> KTNENVISFFDSTDAETQNHDVLMKGCGEFIVNLRTLLRTFRTITDNWILQANTKTPITDLTNTTDAQGRDYMSYLSYLYRFYRGGRRYKFFNTTPLKQSQTCYIRSFLMPRNYSADEINVDGPSHITYPVINPVHEVEVPFYSQYRKIPIASTSDKGYDSSLMYFSNTSTTQIVARAGNDDFTFGWMIGPPQLQGETRSVVP;> KPRNQQQVCPLQNVPAWGYSLYKGIDMSVPLAYDPNNELGDLKDVFPSAVDEMAIGYVCGNPAVKHV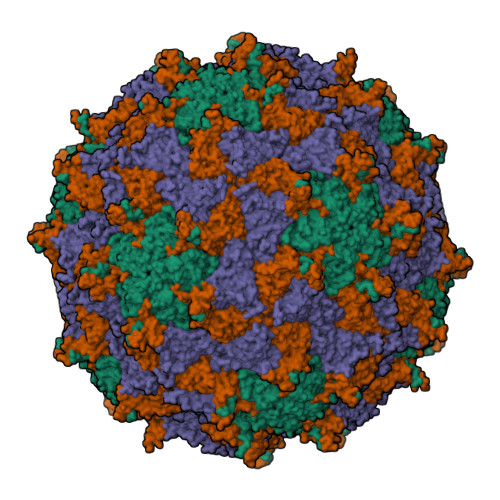LTWKTTDAIQKPIANGDDWGGVIPVGMPCYSKSIRTIKISETENRETEVIDAAPCEYVANMFSYWRATMCYRITVVKTAFHTGRLEIFFEPGVIPVKPTVNNIGPDQDQLTGAVAPSDNNYKYILDLTNDTEVTIRVPFVSNKMFLKTAGIYGANSENNWNFHESFSGFLCIRPVTKLMAPDTVSDNVSIVVWKWAEDVVVVEPKPLTSGPTQVYRPPPTASAAVEVLNVELQ;> ELASSTSENSVETQEITTFHDVETPNRIDTPMAQDTSSARNMDDTHSIIQFLQRPVLIDNIEIIAGTTADANKPLSRYVLDQQNSQKYVRSWTLPSTVLKAGGKAQKLANFKYLRCDVQVKLVLNANPFVAGRMYLAYSPYDDKVDTARSVLQTSRAGVTGYPGVELDFQLDNSVEMTIPYASFQEAYDLVTGTEDFVQLYLFPITPVLGPKSESESSKVDISVYMWLSNISLVIPTYRMNPD>[2x]MGSDKIHHHHHHMAQGTLYIVSAPSGAGKSSLIQALLKTQ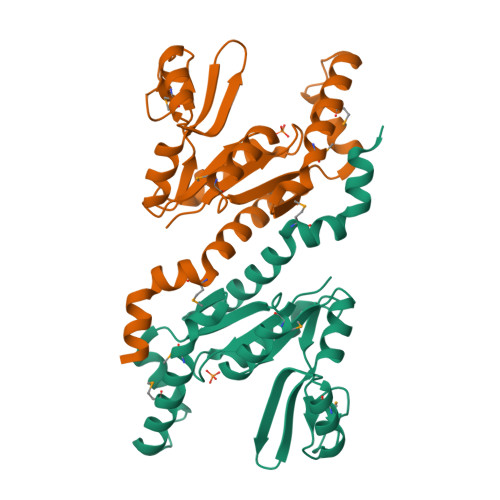PLYDTQVSVSHTTRQPRPGEVHGEHYFFVNHDEFKEMISRDAFLEHAEVFGNYYGTSREAIEQVLATGVDVFLDIDWQGAQQIRQKMPHARSIFILPPSKIELDRRLRGRGQDSEEVIAKRMAQAVAEMSHYAEYDYLIVNDDFDTALTDLKTIIRAERLRMSRQKQRHDALISKLLAD> LPAKENEGCIVSVNSGKRYCLPVGQRSGYSLPDWIVGQEVYVDSGAKAKVLLSDWDNLS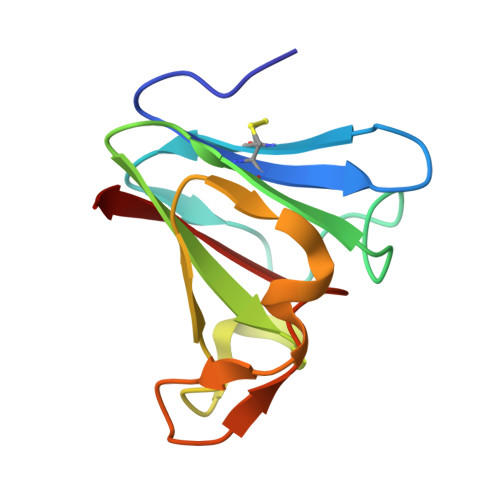YNRIGEFVGNVNPADMKKVKAWNGQYLDFSKPRSMRVVYK>[2x]MGSSHHHHHHSSGLVPRGSQSTSLYKKAGLMISAGDFKNGVTFELDGQIFQVIEFQHVKPGKGAAFVRTKLKNIVTGATIEKTFNPTDKMPKAHIERKDMQYLYNDG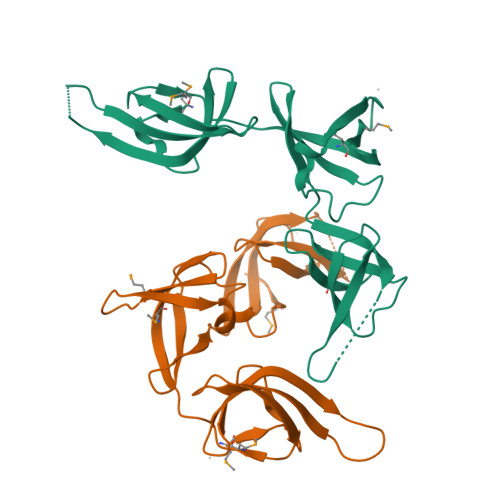DLYYFMDTETFEQLPLGKDKIGDALKFVKENEIVKVLSHKGNVFGIEPPNFVELEVTDTEPGFKGDTATGATKPAIVETGASIKVPLFVNKGDIIRIDTRTGEYMERV>[4x]MSVVGTPKSAEQIQQEWDTNPRWKDVTRTYSAEDVVALQGSVVEE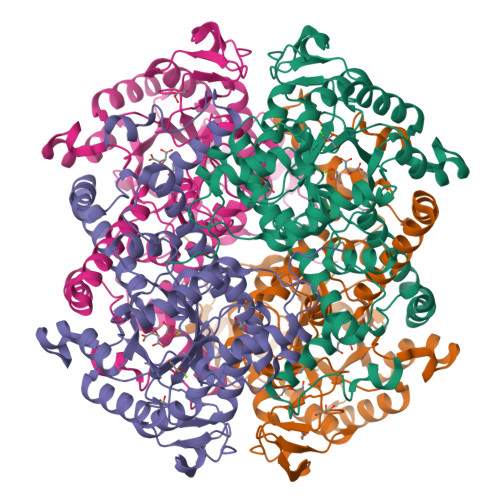HTLARRGAEVLWEQLHDLEWVNALGALTGNMAVQQVRAGLKAIYLSGWQVAGDANLSGHTYPDQSLYPANSVPQVVRRINNALQRADQIAKIEGDTSVENWLAPIVADGEAGFGGALNVYELQKALIAAGVAGSHWEDQLASEKKCGHLGGKVLIPTQQHIRTLTSARLAADVADVPTVVIARTDAEAATLITSDVDERDQPFITGERTREGFYRTKNGIEPCIARAKAYAPFADLIWMETGTPDLEAARQFSEAVKAEYPDQMLAYNCSPSFNWKKHLDDATIAKFQKELAAMGFKFQFITLAGFHALNYSMFDLAYGYAQNQMSAYVELQEREFAAEERGYTATKHQREVGAGYFDRIATTVDPNSSTTALTGSTEEGQFH>[2x]KHSLPDLPYDYGALEPH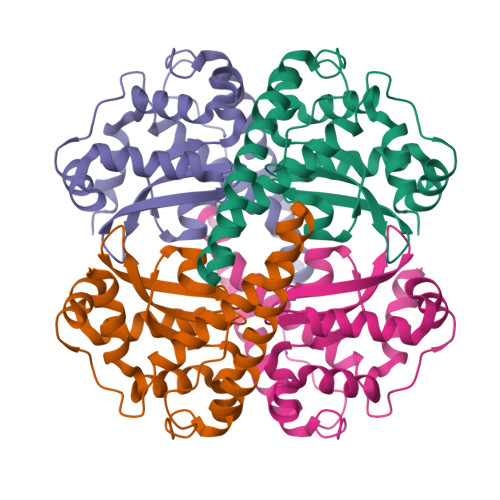INAQIMQLHHSKHHAAYVNNLNVTEEKYQEALAKGDVTAQIALQPALKFNGGGHINHSIFWTNLSPNGGGEPKGELLEAIKRDFGSFDKFKEKLTAASVGVQGSGWGWLGFNKERGHLQIAACPNQDPLQGTTGLIPLLGIDVWEHAYYLQYKNVRPDYLKAIWNVINWENVTERYMACKK> HKVIKNETGTISISQLNKNVWVHTELGYFSGEAVPSNGLVLNTSKGLVLVDSSWDDKLTKELIEMVEKKFKKRVTDVIITHAHADRIGGMKTLKERGIKAHSTALTAELAKKNGYEEPLGDLQSVT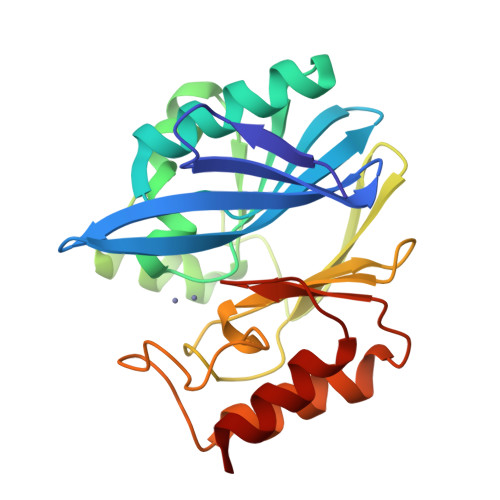NLKFGNMKVETFYPGKGHTEDNIVVWLPQYQILAGGCLVKSASSKDLGNVADAYVNEWSTSIENVLKRYGNINLVVPGHGEVGDRGLLLHTLDLLK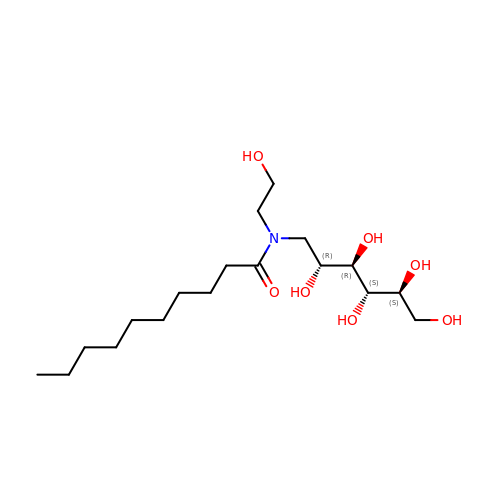HEGA-10 | C18 H37 N O7 | ITEIKACYSCODFV-ATLSCFEFSA-N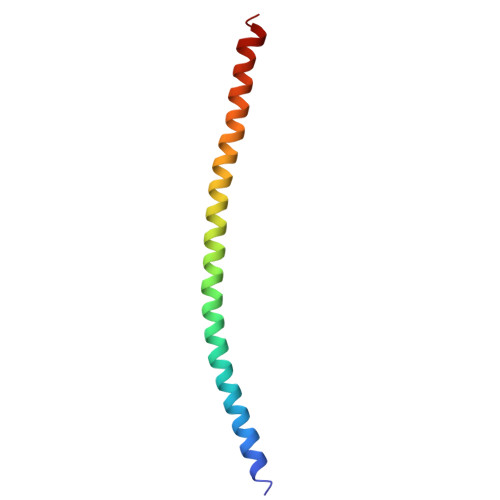> DVSQKIKDIDDQIQQLLLKQRHLLSKMASSMKSLKNCQKELISTQILQFEAQNMDVSMNDVIGFFNEREADLK>[4x]MAAAAVSGALGRAGWRLLQLRCLPVARCRQALVPRAFHASAVGLRSSDEQKQQPPNSFSQQHSETQGAEKPDPESSHSPPRYTDQGGEEEEDYESEEQLQHRILTAALEFVPAHGWTAEAIAEGAQSLGLSSAAASMFGKDGSELILHFVTQCNTRLTRVLEEEQKLVQLGQAEKRKTDQFLRDAVETRLRMLIPYIEHWPRALSILMLPHNIPSSLSLLTSMVDDMWHYAGDQSTDFNWYTRRAMLAAIYNTTELVMMQDSSPDFEDTWRFLENRVNDAMNMGHTAKQVKSTGEALVQGLMGAAVTLKNLTGLNQRR;>MSCAGAAAAPRLWRLRPGARRSL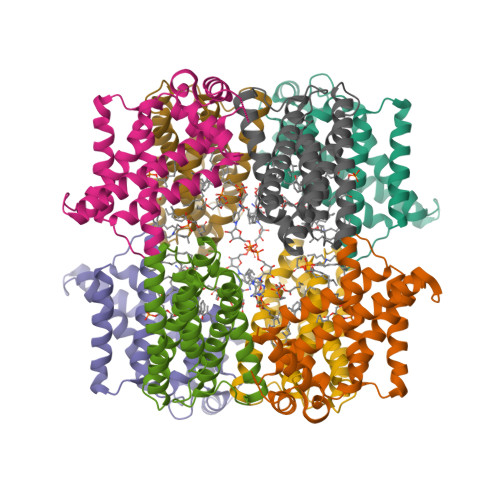SAYGRRTSVRFRSSGMTLDNISRAAVDRIIRVDHAGEYGANRIYAGQMAVLGRTSVGPVIQKMWDQEKDHLKKFNELMVTFRVRPTVLMPLWNVLGFALGAGTALLGKEGAMACTVAVEESIAHHYNNQIRTLMEEDPEKYEELLQLIKKFRDEELEHHDIGLDHDAELAPAYAVLKSIIQAGCRVAIYLSERL[4x]> MNCRSEVLE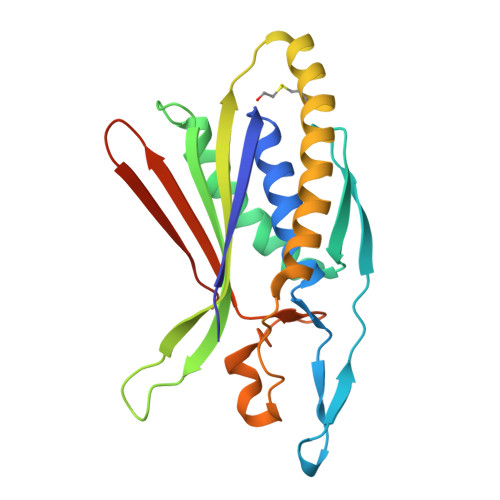VSVEGRQVEEAMLAVLHTVLLHRSTGKFHYKKEGTYSIGTVGTQDVDCDFIDFTYVRVSSEELDRALRKVVGEFKDALRNSGGDGLGQMSLEFYQKKKSRWPFSDECIPWEVWTVKVHVVALATEQERQICREKVGEKLCEKIINIVEVMNRHEYLPKMPTQSEVDNVFDTGLRDVQPYLYKISFQITDALGTSVTTTMRRLIKDTLAL>SGISLDNSYKMDYPEMGLCIIINNKNFHKSTGMTSRSGTDVDAANLRETFRNLKYEVRNKNDLTREEIVELMRDVSKEDHSKRSSFVCVLLSHGEEGIIFGTNGPVDLKKITNFFRGDRCRSLTGKPKLFIIQACRGTELDCGIETDSGVDDDMACHKIPVDAD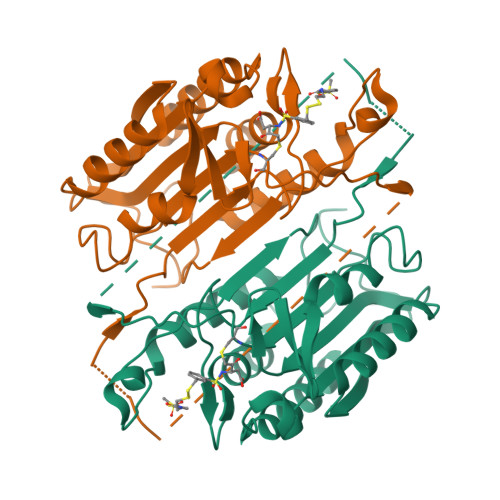FLYAYSTAPGYYSWRNSKDGSWFIQSLCAMLKQYADKLEFMHILTRVNRKVATEFESFSFDATFHAKKQIPCIVSMLTKELYFYH[2x]>RRGLLPNHIWQGDVTHYKYKKYKYCLHVWVDTFSGAVSVSCKKKETSCETISAFLQAISLLGKPLHINTDNGPAFLSQEFQEFCTSYHIKHSTHIPYNPTSSGLVERTNGIIKNLLNKYLLDCPNLPLDNAINKALWTLNQLNVMNPSGKTRWQIHHSPPLPPI[4x]

IN first catalyses 3′-processing of the vDNA ends, exposing reactive 3′ OH nucleophile groups that it uses to attack a pair of phosphodiester bonds within target DNA (tDNA), resulting in strand transfer. In this work, we determine the three-dimensional structure of the deltaretroviral intasome and characterize its interactions with its host factor, the PP2A-B56γ subunit. The deltaretroviral IN host cofactor B56γ14, as part of the heterotrimeric protein phosphatase 2A (PP2A) holoenzyme, interacts with a number of chromatin-associated proteins and potently stimulates concerted integration activity of deltaretroviral INs14.

To aid the interpretation of the cryo-EM map, we generated a high-quality homology model of the STLV-1 IN/NTD using the SWISS-MODEL server, and determined a series of X-ray crystal structures spanning the catalytic core domain (CCD) and the C-terminal domain (CTD) of HTLV-2 and -1 IN. While the canonical IN/CCD dimer observed in crystals could be docked directly into the cryo-EM map, the CTDs could only be docked as monomers.>MRFSHFLKYNAVPEWQNHYMDYSELKNLIYTLQTDELQVGDNEEGFGAGKSSNITDRFKNKFSFKNAKEDTSSGMNKDAGIVEETIELRELPTAQTVAAKPSPFRRMKEKIFYKRRSSSASSVSSTANENLQLDTYDTFVGDLTAEKQKVDDFYKRTEAKFYDKFDALVKDLKKIGVIEYDIDDDTLFNEPIASTNDEVPPLDLDDDEDDDEFYDDQSNIEDNTALLHHSQYNIKSQKKSLLKKSIVNLYIDLCQLKSFIELNRIGFAKITKKSDKVLHLNTRTELIESEQFFKDTYAFQAETIELLNSKISQLVTFYARITDRPHNISHSKQELKSYLHDHIVWERSNTWKDMLGLLSQADELTPKETEYNANKLVGKLDLEYYRWPLPRPINLKFTSINNVALPKLFFTKKAYKIYFIILVTGLLLGIKTFNDAAQHRCMALVECVAFLWASEAIPLHITAFLVPLLVVLFKVLKTSDGAIMSAASASSEILAAMWSSTIMILLAGFTLGEVLAQYNIAKVLASWLLAFAGCKPRNVLLMAMCVVFFLSMWISNVAAPVLTYSLLSPLLDAMDADSPFAQALVLGVALAANIGGMSSPISSPQNIISMSYLKPYGIGWGQFFAVALPSGILAMLLVWILLFTTFKMNKTKLEKFKPIKTKFTVKQYYIITVTVATILLWCVESQIEGAFGSSGQIAIIPIVLFFGTGLLSTQDLNAFPWSIVILAMGGIALGKAVSSSGLLST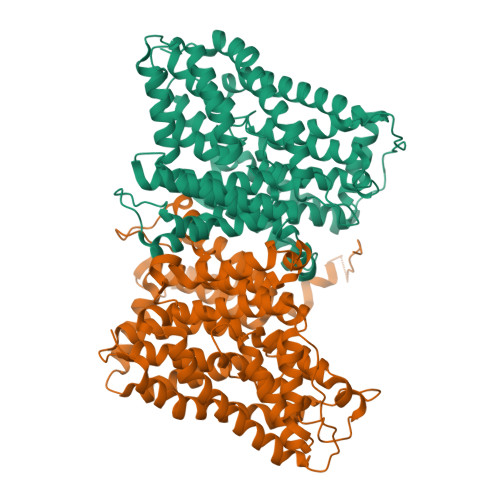IAKALQKKIENDGVFAILCIFGILMLVVGTFVSHTVSAIIIIPLVQEVGDKLGNPKAAPILVFGCALLSSCGMGLASSGFPNVTAISKVDRKGDRYLSVMTFLTRGVPASILAFLCVITLGYGIMASVVKGNATSA[2x]>[12x]ELSAVNDILASIGEPPVSTLEGDANADAANARRILNKINRQIQSRGWTFNIEEGITLLP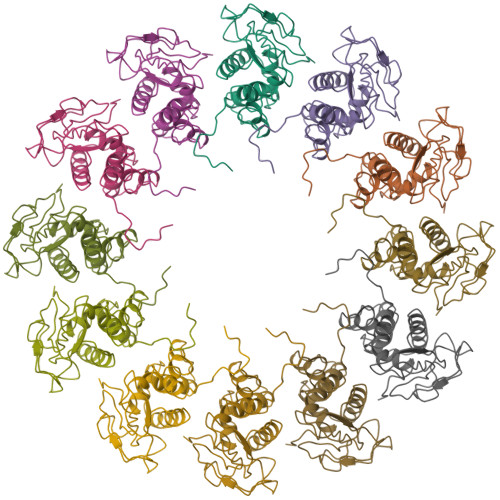DVYSNLIVYSDDYLSLMSTSGQSIYVNRGGYVYDRTSQSDRFDSGITVNIIRLRDYDEMPECFRYWIVTKASRQFNNRFFGAPEVEGVLQEEEDEARRLCMEYEMDYGGYNMLDGDAFTSGLLTR>MGSSHHHHHHGGGSENLYFQGCSDIWALQGKSTETNPLYWLRAMDCADRLMPAQSRQQARQYDDGSWQNTFKQGILLADAKITPYERRQLVARIEALSTEIPAQVRPLYQLWRDGQALQLQLAEERQRYSKLQQSSDSE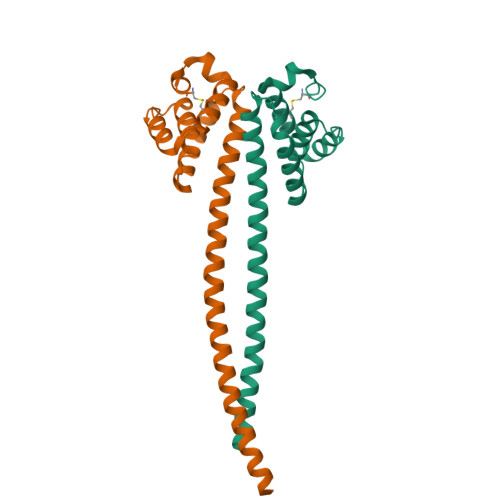LDTLRQQHHVLQQQLELTTRKLENLTDIERQLSTRK[6x]> MGNTATEFDG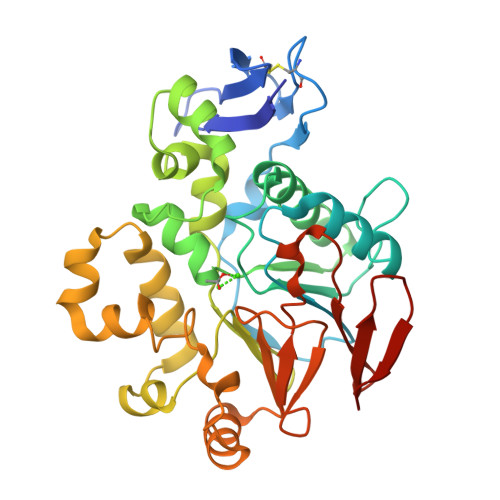PYVITPISGQSTAYWICDNRLKTTSIEKLQVNRPEHCGDLPETKLSSEIKQIMPDTYLGIKKVVALSDVHGQYDVLLTLLKKQKIIDSDGNWAFGEGHMVMTGDIFDRGHQVNEVLWFMYQLDQQARDAGGMVHLLMGNHEQMVLGGDLRYVHQRYDIATTLINRPYNKLYGADTEIGQWLRSKNTIIKINDVLYMHGGISSEWISRELTLDKANALYRANVDASKKSLKADDLLNFLFFGNGPTWYRGYFSETFTEAELDTILQHFNVNHIVVGHTSQERVLGLFHNKVIAVDSSIKVGKSGELLLLENNRLIRGLYDGTRETLQENSLNQ SPHINGOSINE | C18 H37 N O2 | 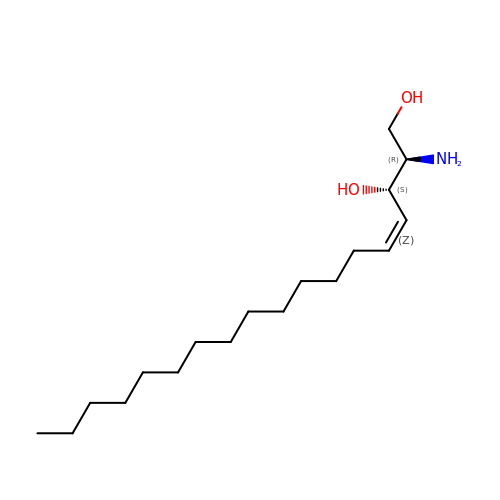WWUZIQQURGPMPG-MSOLQXFVSA-N> YVD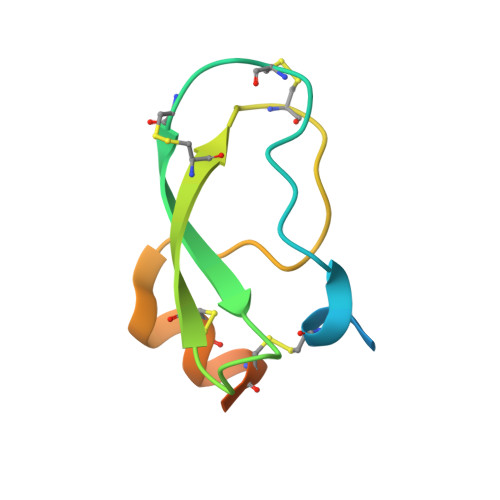YKDDDDKEFEVCSEQAETGPCRACFSRWYFDVTEGKCAPFCYGGCGGNRNNFDTEEYCMAVCGSAIPRHHHHHHAAA>GPLGSMKQMGSMHPVQVIAVTGGKGGVGKTNVSVNLALALADLGRRVMLLDADLGLANVDVLLGLTPKRTLADVIEGRCELRDVLLLGPGGVRIVPAASGTQSMVHLSPMQHAGLIQAFSDISDNLDVLVVDTAAGIGDSVVSFVRAAQEVLLVVCDEPTSITDAYALIKLLNRDHGMTRFRVLANMAHSPQEGRNLFAKLTKVTDRFLDVALQYVGVIPYDESVRKAVQKQRAVYEAFPRSKASLAFKAVAQKVDSWPLPANPRGHLEFFVERLVQHPATGSAV[2x];>GPLGSLFRSLVGTSRAIQQVRQMMQQVADTDASVLILGESGTGKEVVARNLHYHSKRREGPFVPVNCGAIPAELLESELFGHEKGAFTGAITSRAGRFELANGGTLFLDEIGDMPLPMQVKLLRVLQERTFERVGSNKTQNVDVRIIAATHKNLEKMIEDGTFREDLYYRLNVFPIEMAPLRERVEDIALLLNELISRMEHEKRGSIRFNSAAIMSLCRHDWPGNVRELANLVE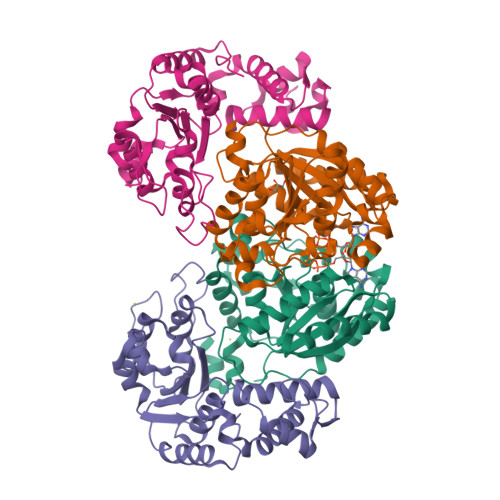RLAIMHPYGVIGVGELPKKFRHVDD[2x]>[2x]MGSSHHHHHHSSGRENLYFQGMDSYSITNVKYLDPTELHRWMQEGHTTTLREPFQVVDVRGSDYMGGHIKDGWHYAYSRLKQDPEYLRELKHRLLE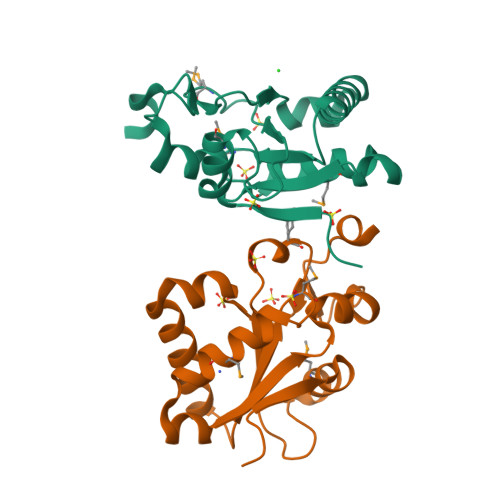KQADGRGALNVIFHCMLSQQRGPSAAMLLLRSLDTAELSRCRLWVLRGGFSRWQSVYGDDESVTAGYLPDLWR> UCGUUGACAGGACACGAGUAACUCGUCUAUCUUCUGCAGGCUGCUUACGGUUUCGUCCGUGUUGCAGCCGAUCAUCAGCACAUCUAGGUUUCGUCCGGGUGUGACCGAAAGGUAAGAUGGAGAGCCUUGUCCCUGGUUUCAACGA

SL5 is the largest and most complex structural element in the 5′-proximal regions of βCoV RNA genomes. We further determined the 3D structures of the SL5 elements from these representatives using single-particle cryo-EM, which revealed remarkable structural similarity despite the low sequence conservation and variable lengths. All four structures exhibited a T-like shape, with the topology of the junctions featuring the SL5 basal stem positioned almost at right angles to the coaxial stack of SL5a/SL5b stems. Overall, the SL5 elements exhibited remarkable global structure conservation, despite the divergence at the level of individual nucleotide residues and their base pairs.

Cryo-EM single particle analyses generated high-quality 2D class averages and maps at 7.1, 6.5, 5.9, 6.6 Å overall resolutions for OC43-CoV, SARS-CoV-2, MERS-CoV, and RoBat-CoV, respectively. Our results provided detailed insights into the SL5 3D structure, revealing a 4WJ architecture in OC43-CoV, SARS-CoV-2, and MERS-CoV, and a 3WJ in RoBat-CoV. In SARS-CoV-2 and MERS-CoV RNAs, the base pairs at the junction motif were the same. The junctions of SARS-CoV-2 and MERS-CoV were most similar to each other, with an RMSD of 2.36 Å. In SARS-CoV-2, only the SL4 GUGUG motif binds RBM24, not the SL5b version. The last guanine (G252) of that motif in SL5b contributes to a four-way junction. The SL5 stable 4WJ structure might prevent RBM24 binding. Within the SL5 element, the first increases in reactivity values were also observed at 62°C in the basal SL5 stem, particularly for nucleotides 165–170, located close to one of the bulges, and nucleotides 265–269, encompassing the ORF1ab AUG start codon. In a chemical probing of SARS-CoV-2 RNA at varied temperatures, base pairs near the AUG start codon in the SL5 basal stem broke first, highlighting the role of dynamic regions in translation regulation. Volume maps of the molecule across all frames revealed that the SL2/SL3 region (corresponding to the smallest structural feature of the molecule) was occasionally visible. This suggests that the 5′-proximal region of the SARS-CoV-2 RNA genome adopts a dynamic structure, with SL5 as the main stable element.> INTITFDAGNATINKYATFMESLRNEAKDPSLKCYGIPMLPNTNSTIKYLLVKLQGASLKTITLMLRRNNLYVMGYSDPYDNKCRYHIFNDIKGTEYSDVENTLCPSSNPRVAKPINYNG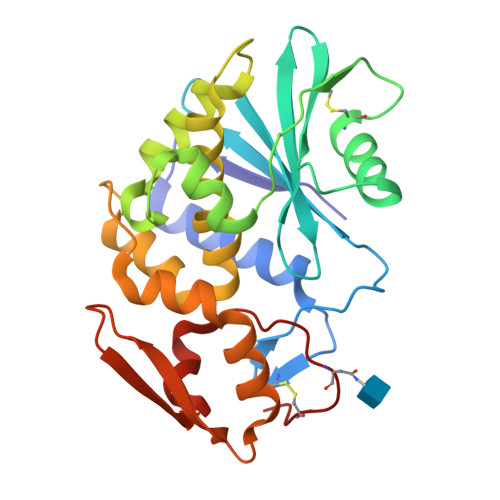LYPTLEKKAGVTSRNEVQLGIQILSSDIGKISGQGSFTEKIEAKFLLVAIQMVSEAARFKYIENQVKTNFNRDFSPNDKVLDLEENWGKISTAIHNSKNGALPKPLELKNADGTKWIVLRVDEIKPDVGLLNYVNGTCQAT> MIVKHLEEIVDTKDDIDTTTWNSRRLLLTKDGMGFSLNDTLIKAGTETLIWYKNHVEAVYCIEGEGEIEVVGGETYPITPGMMYALDGHEKHYLRARSQMRMVCVFNPPLTGAEVHDEEGTYPLLAPITDGSAWSHPQ

While the EctA and EctB enzymes have amino acid sequence-related counterparts in various biochemical pathways in microorganisms, the ectoine synthase (EctC) is considered the diagnostic enzyme for ectoine production. Crystallographic analysis of the psychrophilic S. alaskensis EctC protein [(Sa)EctC] showed that ectoine synthase is a member of the cupin superfamily. By using an ectoine synthase from the thermo-tolerant bacterium P. lautus, we were able to obtain high-resolution crystal structures of the full-length EctC enzyme in complex with its iron-cofactor, its substrate, and its product. The (Pl)EctC protein is a head-to-tail dimer where backbone interactions between two ß-sheets mediate the contacts between the monomers in the dimer assembly.

To obtain crystals of the (Pl)EctC enzyme with its substrate N-γ-ADABA or its reaction product ectoine, we added these compounds to a final concentration of 40 mM and of 20 mM, respectively, to (Pl)EctC preparations pre-incubated with iron. However, crystallization with this substrate was carried out at pH 4.2, conditions under which the (Pl)EctC protein is practically enzymatically inactive. The substrate N-γ-ADABA was added in large excess (40 mM) to the crystallization solution; however, the obtained crystal structure displayed only a partially bound molecule, which resulted in an occupancy of 68% after refinement. The N-γ-ADABA molecule is coordinated within the active site of the (Pl)EctC enzyme through six direct interactions with residues Trp-21, Arg-25, Asn-38, Thr-40, Tyr-52, and Glu-57. First, a direct interaction occurs between the O atom of the acetyl group of N-γ-ADABA (acetamide oxygen) and the iron co-factor with a distance of 2.6 Å. Notably, Trp-21 adopts a dual conformation in the crystal structure of the (Pl)EctC::Fe/N-γ-ADABA complex, in line with the observed partial occupancy of the crystals with the bound substrate. The comparison of the (Pl)EctC::Fe and the (Pl)EctC::Fe/N-γ-ADABA structures therefore suggests that the presence of the N-γ-ADABA molecule within the substrate-binding site of the ectoine synthase induces the reorientation of the side-chain of Trp-21 to provide additional stabilizing contacts to the N-γ-ADABA molecule. As can be observed in the (Pl)EctC::Fe/N-γ-ADABA structure, the water is replaced by the amide carbonyl group of N-γ-ADABA upon substrate binding. The (Pl)EctC::Fe/N-γ-ADABA structure reveals an extended conformation of the substrate within the catalytic core. The distance between the carbonyl C-atom and the α-amino group of the bound N-γ-ADABA molecule (4.1 Å) is far too large to allow a direct enzymatic attack to initiate ring closure.> MKALIGIGLCAALLGGCAALPGRDGPRECSQQLGQEQELQMNMVRDMIREGRLHAALANLESMPPGLLDVREERALILRRIGDPRARAEYQALLETCKAPEAHHGLGLLALRNGDSARAVLELREAARLRPTESRFRNDLGVALLKRGDRVGARFEFITALELQQGGKLPATNLLGLLYLQGDREDAQRLIERLQLDARDIRAAEARARS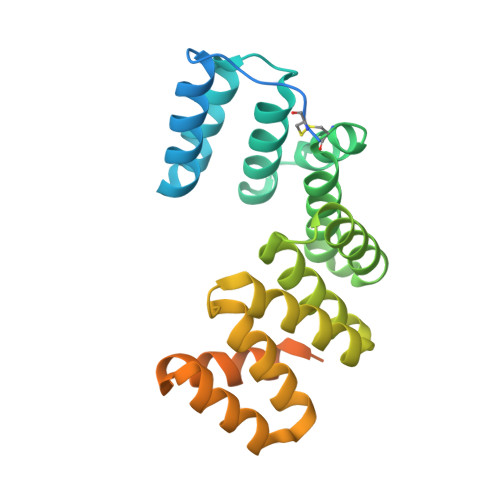WGAVPTPGAAPASDDPLAELPAEANMHTAMANEAPGSDYKDDDDK>GMAEEKKKKLSIIVFSGTIDKLMPVGILTSGAAASGYEVNLFFT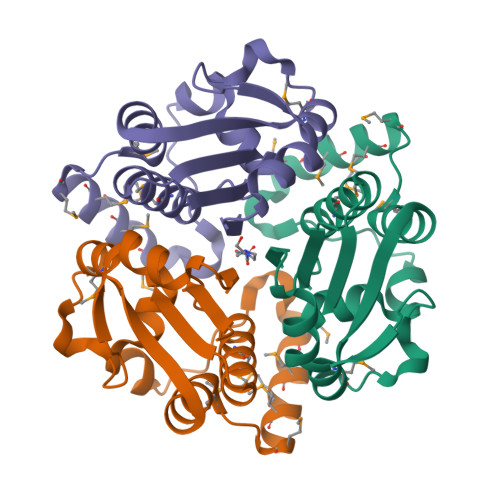FWGLQAITKRSLNSQQPPQIDKNYEQMGPIMMQKMQEMKYPMWHQLVQQAKEIGEVKVFACSTTMEFFGIKREDLAEFVDDVVGVATFLDRAEGGTTLFI[4x]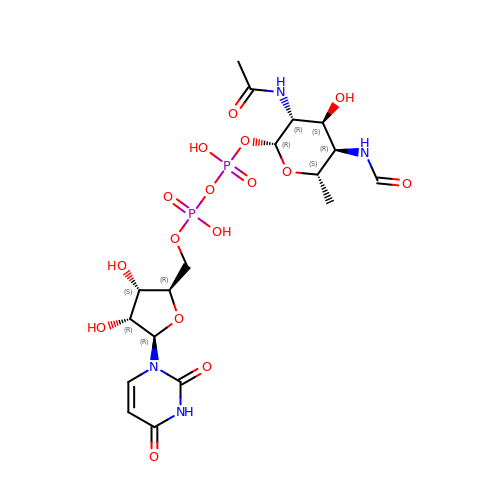(2R,3R,4S,5R,6S)-3-(acetylamino)-5-(formylamino)-4-hydroxy-6-methyltetrahydro-2H-pyran-2-yl [(2R,3S,4R,5R)-5-(2,4-dioxo-3,4-dihydropyrimidin-1(2H)-yl)-3,4-dihydroxytetrahydrofuran-2-yl]methyl dihydrogen diphosphate (non-preferred name) | C18 H28 N4 O16 P2 | MNNFOPXYMSSSNV-XQDVVILDSA-N>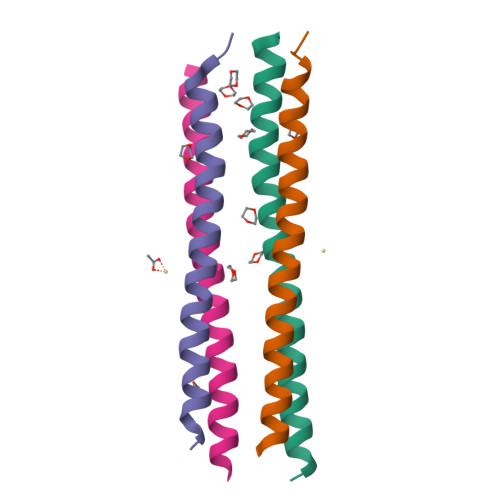[4x]MKQWSEEVERKLKEFVRRHQEITQETLHEYAQKLGLNQQAIEQFFREFEQRK> MHRFRVCALGAAFCVARRWRSGGGPGDRRVRTDWYRCYPSLMEEKDRDMYHCYYPYLFDHGDKMSLYPKIPDNPREWQVEQLQTTYDAIREDKYDAFVRLRAKFPELYQDTYAWDNPPPFGEFNMFYSVRFGMIGVKAFTCKDYDDLGNQFDCTAFWFPDNQIVKHSTRNGDVGTDKVYVGAMNVPVEFHKPHVAAFYKAAGVPVKHVSAGFPVTPDAYAPVGTKLDVRHFKPGQEVTITFQNTDYGYQGVMFRHGFDGGYVWLGDSKWQRRPGCMGAEGQKRIYPGHRMAGQTGASAETYDGVPVWRIDYKNSLIYLPTLIDADVGTYVKFRDTINTKGYTLWNEHRGTPPFPTFIPSEEEDLSKLATDEGQLTSPPLYMYFRDEFAAAQLVTQADVEDAKSAKPATAAPKKKVYDLKKYTEARKKYRKNLQKARKYKLMGVRTRAHEKQQEARRAKILKYKRVKT;> MLRLTQAVLRVQSHQKKRAQHPNAGTRFGRVYNRGFVRYGFGGFGMSVYSSKKDRTFKVMPVPPPPPATTAVEQRDDFADNRGLSATTRTLSPTFRMFALEDGGVLVSHPSHAQIMRWNQRVHTEEGKAANSTVMDEYVNSRIQAIIADNTIENTSLSQWRKAHMWNVIKSHGKLQRRWGTPDFVMGARSTLYNN;> MSRNGELCLQRIIVSYSPNKGNPAMRQFMATHLPEFHRQYPQVKIDIRPRQWPESSITGIYRDGSEKAYSIRFLSSMGINVRFHRLVNEGNDYNHSFSASHLHLQRRSVQGTWNPYLWNYEGTRARHKPPAQWSRKLTEKEWDYYVQQYGAQMKAEEDTIADRVRRYTDIPEASTEEVNQRWKEHVMPRLQTDLEYNLSHWKKQHRTGAGRPAPPTLNEYSLFSVPDHSSLGQDAIDMLRRREAQREEDWWRERKGQLKPPE;> MQPRRMAGHFNPTPQANSLAATHYAHTPELRHMADGAAMSLSGQRIPLLKPTLSKWSRQLRSDIYDELLKLPLRYALHDFRTLQAHIHAVPATATNASCTAAAGERLPPGVYHASSGLSSASPDAPAYYAVAGRDSAVGYAPPLGPADPVDVIPFFVHRSSNGHLPGKVYSMNAKTLMPAFYMRIQNIEGDMFRFEEELMKIFPTKKIFVRSHSVYVYNVNLDGRAVLHHWLLGLGF;> MTAPASHYTFANLKKLGLCAPQVALSRQPRLRPHVGHLNGLVYPLPYYAMWRGNHDKYTYNQATPARWGEGNTNTMYHQHYAHAKCPTDYGRGGREFQFLSVKRGKLKRKPLPTVQYVDPNSKPQWVFKSWHNPLSAPSMWEREVQYPEHTPAHTGAKRPLAVVAPKTSHKHLFLMHMEKVTVTVSPLLFGYGHTLQKAALDFYRRGLSARSPFPSDKMFLYYSIDHITPKIEVTWLDGSVYVPPLIEGVKAQDLIQMVMEQAWLAADRMSAEGRVLNPIAIDDYKWEQLIAFKQKRAKGAEAAKGGAKKK;> MLRRSPVPRRYRTAWRELLHPLPVWARRQQWLKRDTVEMNEAILREPYYRIKTFAQPAAFVSPRVSESAAHEPDTQQSSRYGVDRQLRGPRRAVSPERLQELREQLQFVGSIGPKVPPAAGAGTAYQDEYGTRLRPRYPQSWDTVPPHQPSRSEI;> MAFRGSSARLAATPGVGIAPETTPVKYVPEMLNIQNAKWWNGRGKPVYRSTYNEKSWLEKARWGAFTKGSRPVMRQRYSAAALKEALEMVPEGFETCDVPRPPQRIRAQSEGVVGRWYTNYWTLHSVRYQCQLAGVEWQFGERQRPRTNYDEPHMYTDFEETKAIRDYRSRWINVNRSLVGMSRRMKESEEEARYLHFKKVQDTFWSNRKVLVNRIKSMHNQGTLQSAKDLPIKTINIKAFLAE;> MHLHISSIPHRNSNNSKGGVLDATGPMLSAKRGALLLQAYHRPGEVISYKAGDYHLVPKKFTVGKRIAVRSYLDRNRTELSDRTFMPQKNWFRPYDLQDGCFDRDHERLSYRFYNLETKVIWKAFDTPELIGMLLHDETVKGNSGMYAPDMLDAALHYTREARYWRCIGITKPFYDRNTLRAHCWEDNGLQVGTLVMSQAMRHALMDLERAVRRKELGLEPNYLWDRWGPIGFIDGARADYLPRFEHNPYVDPDGVDVTEIDVLPFNTHEQIRERYRDFIEPDTAPFEEVFRSPSHGSLTTLADIPNASVVALYKDLKLKAGTPVAGDAVELAPADVRTLFYLSANPEWRAVADGKASWEEVVDAMQPVQAELDEKIDAARLLQNTRHNAERVRAFFEEKCGFHDFMYTPDKTITAAVLCYLTELRRICTETAWGAALAKCLTDMERVQGMGRDAFLVYRHIEDAILDKKRRLWAGRFAGESHEESTLDYLLENFGRRAERPRNVGTTGVEFDREQEPIGRQVQRRVLDSDKANKLAEIRRSRGKMWSKKRSVFDALHEKQLQNFNYGVH;> MCTRVFDVSQRFILLVSLPPLSLSLRPSCCSRKAATRRRRSTASVLLATDALSLFVRTHYPSPLLFLLLPNFPLPIHSPRKQMRAAVGAVLQPSSSVGALRCQARFITR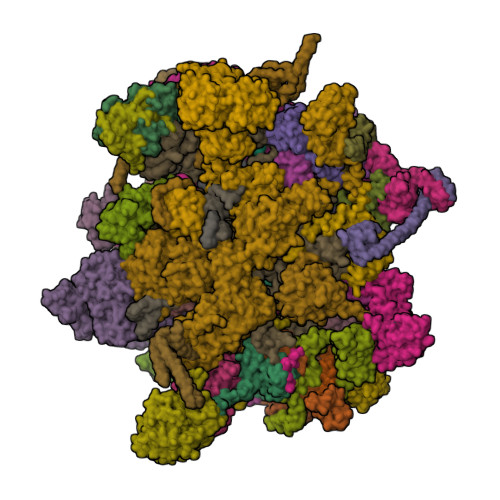LYTSYFKGELFPNQLARPLERLPRGVSLAAARKGQQAAAPSSSGSGNPATTASLDVVTWGDVDSTDLVHANEQSRAVAPQAGLAPRRPYVPLGEVAKLELQGDYLTEGGLHQEALEYYGVVAKAYELAYPKDHPQVAGIRLKLAGAFRRTGRLTSSKANCEAVLQMLDSAVQPPLELIVEALFELGLTSEAMSDAAAGTVFEEAVALVDMFHNSGQSHKMLRLLPRLGRRFNLNFEEKFVYFSPFDYDRVFALADQCLERAEVFYQARNDRAGVMRVLQQRKELIDKKFFNMRDFAGRIHTMRGHWKRRAQVLTNAPTPDELLRYSPTIHQVYRDFKYELNAPIGREKEVQPGVNRVVHDMGNPYRRSGVRSQRMFRDAEKNFEKYIRADAFEA;> MLSSAHRAAFARPTATLWASARSFGAGPTRLLLGLEQVQDVPTSTDRKPTGMHRGPGKRQTAPKEAAQYQFIKKWDLQMRETWDELEPFKGLPKPKVQFGNEAAEVIWPYALLLENVIKVHPYTKSIYVYYSQRQSTPLGELAARVAKRVSQAYLIPITFHNSHVYVEAEMLLEYSETPWVVVHCLDGTHKLIPVKPQAGQTVKEGAEEVLNGIVSACNEIGSAVKNPKEVMRLLSERPLQNQYVRVNYQWYGDTPEERMSHLVKWDYEPEEVVPQLRNRTQHVLDWMNYDGNLPTHNSVRVNIHREAARMRKPNVSAGPKTFFNSSGSRANARTARFDNSRSSQS;> MLRRTEIALKKGWTHNPGHTRRGGKNLAWRPKISDAKLSQFVPLALVHPRRHPNNWQERQFNALGYTKWPKDIGFYNAGDNFEVTPEAAWRLYVHARDEPYWGKLHCEKTIITLLPVVEKAPKENMERVLDVFRHYLKRYGADHYIYNAVMQAAAFAKNYEQAEQLFKEMETLGLEPNAQSYVNMMLAAKLCGLPPEKSEAYFKRAVKDGAMQSVMRMDTEFRMWMDQLDRLGSFTASSGYLSVNEEGAKPMPRDMWAIWGWHRSESKFISRRDLIMQQVRARVHSGKELVGTVYTKTRRQPWAKFNGMLRHDYNGPSYRAPTIFPDAPEYTNEAGHKAF;> MLQCTALVLKSQHKNVLRKGRPHMQKYKELNRWQREAQGITKWEQGHSHRPQPYVERFNPEGAGLTRGTSAYAWKWWHTQYPWLPNVAPADYVPPSPRGIRPAAWDDEFADVVLSMSDEEIQSYLLDKLTEVIFAETQRDGYELRRLDFEGKPLTELPERRIIENFVFEEETLRERVLDRVVEGVFRLVPTSTDRLELKSVANIIDFVLTHVTVARKPLQHEIPEAARTVMRSHPLQPQLGFVHALPTDNRDAVVQEWERMHHLDWQFGKAVYEPRSAENERGNLTWLREVRHHEAREAFQADVDSGEARRRHMAKIKAAAQVPHTGTTSQ;> MQRCLARLFQAGVHTPHGSRYNAARMKNWPVQEVPQNFNFTNEQRFKAKAVPRDTGKIPRDFLLSVLYRNQPCEVASLWEHCLHDPQIVLDSKRHLREVLQQARAEGFVSFEKDAVTDRWVCHLTRERFEEVRALVGARAEAQDLYSGLRGASATETSAYSESFREMNEDTKREHFRLLSEQVADTTTHLRKFQRMEMDYLPYTDLNGKVNFMWWYEMSDTRDATALPEAAAEGSPKLSE;> MLRWSRLLREMAPELQLEYIPIIFTRTILGPQGGFAGEERLIKREVAQKYMSEGNAVTPSAEFHQGVWCYNPDSEQYDRFVERNAEFLDFAARKRQWLDVYWRVNTGYLLFGRQSWGQGWLLNCPLRKKDIAQKLWEQYKVRVDPRLIEFREKDRRTGIQDLGHNWCWLYLPGAEELAIDREVYDNKRVKVRMHIRKMSSYGALY;> MRRLPLFCRRPSRCCGATASGSGSSSAAVLAASAAPSVLVLAARGIATSGRVTNEDRRWWLVHLECAPDVTPGTFVSWLDCCGTHTTKKLIERNIWTIEQVAELDSDRVDELKYKEGCLKMDVVWEHARTIITPLKQREVSGGVESQLQSRILELRKKRELERQRELLARERATVSDKREETLRRLRESVAAKKAALRKKLDEQHGEATPAASESASTEAHRGTAEAAVEDEAVGNIVDRMSGGNPPRA;> MRPSALCLGGFTMKYKRGTGLWDEDHVNDFDANKYLSARSTMRWYYGMERLQTRNNMNARRATQSYNNNMGLHHSGRGAFERELERRGIQVDKYPLTTTTGAARVAEMVLLRRQELEAHAKKAMESQRQARRRDAPSEWYDETEGPLNPRFLASMQSNYTQVITELPSSPVTGRRELPGASFA;> MMLQHTSLLCRKALQSYPVPPRARNYERRWSSSRTNPYNRMFWRTVLNEDFARPSFWVSDFRHKYLAKHGMDYQGRVPASPAPGMYQGFSDVHKILANHPKPQRESRHLPVMPMTPRVVFEHAQEKRIDYAKKMHRDRRLVEQLRTHEFWGWYMKLQRVRGRWCKEHGVSSRGVYGPAVDAAELWG;> MFQRTCTPRLLACTSALLKRSGKPSDLPDYKQVYLPYDTAPTKTELDRERRKFMHAYSGRMEHRKMVEVKDVPQNMYTYGKEGMSIPISIFKDQADPVIGPEWTYPGIFENKIVAQHWYMEELFDREKSNTFESPWQRQVLDNQVKRRLGKVAWRMSMLNIKTIDIFHKERGASKRPGAGDTKAPATPAGKK;> MSSGAVGRGSFHSVVAGANPRRIPTYYNSAYELIQLHRAHREVTRNFLVRDKVFDNKFPGCSLANGLFKMVPNKRGNFHTRELTESIRHRTIWGQRIQQQRTINAAILEDATKVLSPAQMEDRFSYRTPDAAAYFSPQEYTAANNWPNYWQHPTEKHVVPKPRWRREPELGGITRVRDAVATPIADY;> MYFYRRIPSLASKMNHMRQFSLPRSSAAIIMAASTAALAVPCRAMHGKPASGHKVRTQHSRRWWMQSKAHHLTAVPHEEARSRPHFPAYTEDVDQPMVVPDGVCCFNCDKPIDGDDINSYVWVPSGNARVPTTQGYFFHVKCFKCWNCKYRIIHNQFYSKDSRAWCLSCALGRDIRVPTRRWHTSYVNTHRTGSRLTGQFFPRHRHQMEFLFSPKE;> MLRFTQVIRKNPVVFKQGQGMFSHQLKRILNKKSLHKYNWDPLHMYDPRKLVHANRYVDHDTYEEKYDPHWEHNAHLVPDQQFYNIPVPKEYKDAYWWRDLQARRVQCPTEWVHFRMHTKDKLKYDFQDLAFRKKFEYSYEDVVANAKDMCS;> MYDSRSSGVHDVAPRDGVDFMYEGPQQVLPGAHPLPLFHPDNSVTRPPVSPYLPSPQRPHPYFTTELPELPHFQTTRPIVYTVGTMKQRIVAPVFDLANNVTHTRELDPFIFGFYPETEEMAKNLSYWLVRCQNFSSKWDYENREIWRKAKKNWPNTGMGMARVGDRKNHAHPWGAHSKPVKPWNLLMPTMDVKTWSKSNRMLVTLKMLQGKLQIVERLTLPEPTQEAYLQLCRTMGWDVRHKGGGALFMDGGSRLTPSSEYDRAFFFGSFFNGRNKLVRPTLLCDEPYDYNRTSSKARTKGPKGQKNPIPINRFNAYDALTHDTLIITEGALLQLEDEMYTHKLAMLPPHIRAQLPERGFLDSEVLGDVPPALQTVQMEAAARTEEAEQAMYAPYYDNPYHPWQDEGEASYAVDAVEGTVQRYIKSRKTSWAMLS;> MAQWIPKTAWKVSNLNKRYGAPYVAKGYASLDPRCSLDAYSSFQQTVTSADMKKALLSIDSTSSGALVIDVRSEPERRLRPLLSPAIVALHPHDILSGAACPILPSNKERAEMFVVASEAQRAVNACTALRRWGFSRVTAVSVDAVSEAIAAVQKPADAATSSSTKS;> MLHRSCVLVDSFKEHYHRVHLPRRLALQRYIKREEARLSRHKGKAVAAAAAAGVQPGEVAYKYNRWWVSNDHEFVHQFAFVEDPDVTREKRNTLPLVTKENIWKEPQQTFFLPFAPFVRVVDYAKDPDTKFLKPVNIPRWKDYMQRTKPIVPRTWY;> MLGGLRPLAAATRRTVGGALVSPALITPSRALSVRTEDFFSKEAVSHARRVSWAPHTTEKKVGAFAKLSRSNFNDPLPVSFQSEPYFEEEIEAYRAHHRPDVYVYKYNVSPTHLSLRE;> MRRTVRALYNSFERGWKDKTVHPLDRRGRFNLDEAAAELQLDEAYVASLYKPLHYTYSMKGQRYPAEQGRTSRPGSLAASRDRMFPLYRRNYKLNRELRVLDHRRISTD;> MLARYLDPSVHPLRVGQVVAYDYLHAAKTWQWTLGTVREIKDYTAVVQQWGLHTGDIDTLRSILLKEVDTENGRMKNYHDMLAIAREKLASIRRSNEDRVSHVRGHFDKAREKVELIDEVDLRKVTAQAAPSPVAVAVLKAVWAVAKCDPTAVEFYEWADVQLEYRKPAALDEIAKTDVLAKLYPSAESLQQSLEQDPKLNYKAAARDSPVVASLHAWVITALAYQQAYNLLAHDKRIQEQNDAIAAAIAGMKACRAKIAKLKDELSSKDTAALPGQVTSFTRTSVLVTIPLSAVISPVNVDTDVKRCVLTKDEVEQIPIDAKITRYAQKQKLAITGSHLLDQYAAATTTHIYVTELEDRLFFFQHYMASALRDAQTAAVDAHQRLAVSLHELEAFRQKRHDAKKARAAEPELADADGVEPSSGPTSSRSPTGRAAPRGQSAAPRGTASQQHKLLGPAYQSIDPATIANEPLYAVTIEEYKAKDAAGERAMDEAERMADEVQRLAVELEDAKAAADKLAEELAAKDEELAAHRQKRHDAQQARASDPALAAADAVAPRSGKGAASPHVGAVQRQAVDPATVPVAPAVIAEEPLYVATAEELQHVRDFADQLAEELEAFRQKRHDAKKARAAEPELADADGVEPSSGPTSSRSPTGRAAPRGQSAAPRGTASQQHKLLGPAYQSIDPATIANEPLYAVTIEEYKAKDAAGERAMDEAERMADEVQRLAVELEDAKAAADKLAEELAAKDEELAAHRQKRHDAQQARASDPALAAADAVAPRSGKGAASPHVGAVQRQAVDPATVPVAPAVIAEEPLYVATAEELQHVRDFADQLAEELEAFRQKRHDAKKARAAEPELADADGVEPSSGPTSSRSPTGRAAPRGQSAAPRGTASQQHKLLGPAYQSIDPATIANEPLYAVTIEEYKAKDAAGERAMDEAERMADEVQRLAVELEDAKAAADKLAEELAAKDEELAAHRQKRHDAQQARASDPALAAADAVAPRSGKGAASPHVGAVQRQAVDPATVPVAPAVIAEEPLYVATAEELQHVRDFADQAAHDAATREAEVAGTVENLRNELDDVREMNAKLEDEVFALKEQLSDAEDAYKKLAGALVVAEDERQELCDDLEAALDELEQKKDEYDELLGNLEEVQGLLEAADVAGRTAVEALEQRNRDMADLQGELANALDASKENENLRALLDAKEREIDRLKEYNSFWTDTVGTGKQKVTHRLTKIFDGDWTRLMRHRPEALKAAFVIDSSNACHVPGDQIFLVSNSFTRRLLTRTDHCPKCDRLSTFRFMSVSGMVGRMPYKPVDTPGPSYATLYWRKQRSGKIASQPLNEVCNKNEF;> MWRLSRVALQSNRAALYMPYTPVATNPVVYFDITAEGDALGRVSVELFRDVVPRTSENFRSLCTGERGYGQCLLYYKGTPFHRIIPGFVMQGGDILTKDGRSNVSVFGYPFPDESFEGKAGKHLPGTVGMAHSGPNQNGSQFFFNLGRNEQLDRKFVVVGQVLGGWEIVNQVVKLCGSRCGTPVSRAWISDCGQSGGYMAEETQEALQGERAQHVIPGKEVLDLIQPRY;> MRFDNAAPPPPPPPEAAGSTTTSSSTAASALPRVSYRTLPSSMYPKEVSSDFIPFPLPKHDASMGFGPVRLRNVPDIEEARARMAKAAQGPPRGSASTQLQDADGDNAEAASALWAELSGETTATSVGLSTTSVTGASPEDPEALSRPPDAQDEDLVGYHVHRHFPLLDVLGCDRSVNDLLAQFWNRPQREARTATVLDFAATLQRHSNEELTRVLYELSSLFEWDGNGLQFIAAKVLKYGRSYTVSSELTKAFVQLVDAMTVAFVEEQPHRLAESPALLAQVLHFLALVKIMEPNKWYTLNPNAPQNRADYTHPRGVNRTCGHVTTGRALLDFLEDMVTSGHNWTGEAAVDDQQGSLARSPVPQHATNRFTEGWSEDDILDVMAGFSGVMPDGKASSPVLYALLDELWMRWSKVGFVLSGSEQAVRLERLYMLLQVMDMQRDAVLDALLGGQLRAHSTAPSTSTLPTLFCERDDTPPLTLAQSLTQTRGPDFFSAVSRDKRAMVKAAALRLLTASLAKARDDSDAVLHQALVESGTELLQSLTSKSAALSFAQREQFDVITLRAVPHMADVAERLAEQRAEAPFFPLTASAGGLPDTAAVLAHLSSHPAPYIVLCKGRRVHPVRTLVSNLDHVAAVENVFLLHSSGVSKCVDALVAVARRLRSGKDALIVTASCLRALQAAAQYGATEKRRATADRALDIVSYELEAGRAILMPVTDELYLHDAGTYCDEDLMLWTLAAYLARDVPLVKVHTIMSSRSRARNPQHALRGEHSPLTSTDDLYNKSTPLLQALRSKELRAVTHHPVVQRPVRDPPQTLYNVNPIRARFVYRRDKALFDKYHVTARNLAPGFSQGALNSDLRALGFYTPDHPQVPYTPLSELKCHPVPANPPASQ;> MSVFPGLCGDVATTNYRVFLGTLPNLAVEERFLRQVQPVFPWYASRKHVKEQASEFLEIDLASCDPELLLRYTHVYYVRRQLYDELVDRQLTLMETGKAAKVADSALLTCLAQVNAAITPRLQYELHLLQQAKKACRVPRRRELNPDAALEAHDYLCMMRVVEEDVGGIPDAEMQARAYLPREVLEAKVKELAAMIFGDGGSATKGTGAALERKEQKLLQRMIPADYNKVGAVEKLRPVDVTALYRFTGERVCGRPADKPFARALWGHVFRKVGSHPLYLQRASLYWARHSGLDPQSATSAMPADLATAVCVQQALFPALKYRCQYLYTSPDIARQQWRTGHVVPLLRLFPLLGAPAAEDLAAQLVVEGEWAKLGIEADTNLLHDTVLRQLKDMVEQVSALYESDAGAVLKRVEDGAKVLCPSLSERESLTMRGAPEDTSREVSAAAAARVANAAPA;> MRAAPTRLAPSTVASLGRSHCGSQAYHLDAAGAAGWRRRRRLTGVSMTTTHTVAPAVSALPFSLSTARRTYYWPYPENLVPEGATTSPFQSSPVPSVRERIIREYALGPLFGSRTPCCVLGFAGTARDVAACKRDVRRWVARALGKSEADVELGALVQAKEMLLHRSGTDESPRLGDGPGSRPDAEQRRVTRYARLPVQARTLLEVYLPGEEHGEVDAAADADATILAHGYFLQEQLHRHMTTTASSGSDPTGRRDSEDCQPEEPARKMQSHCQGCSEPNDEADVKSSVAALHDVCGVIYCEVPVLDESDFAFDQLCGKEVDDETTERVTDRWTRRAMQQQPQL;> MLRFFRARLAPTTTDAAAKLPAGNPVNKTWFRHNLIIRRKGSYRSRWGNGTEGYGAGVPLSDQVKLHCVDNTNCKHVRLIAKATAERFAHCRVFPAVAHRVSVQRFKGRGGGGEVSRHRVKPGNIYWVCLFTRRQTNTRMSGLQTNFDRNTCIIMNDQRVPLGTRVMYCAGRHVNHKYHLKAVVLANFFV;> MRRRDWCGVCLPAATLHALARRYSEYRSSYTGARSAPWAAPEAAPAYPSARSPFPLERPRFRKTHIEWMLHHGHGDRYGKYGPSREIADFEYADGTPSSISGKRFALKHHQDHLLVQLIRSAAIVERFEEEELLPRIPGTPEQRSWDPEIPLFLEDVDEFGRPPRPVAGNMVARVIEERFAQESGRTPVNLANKHAGEVLEPNTMFATYDPAAFVSDDIKKDVRRPFWSRRRWALSDNFMVPMSPKPKNTIKDE;> MLRRQCVVLSYQRGSWAPGSKHQKHMSLNPTMYLYRFAGPHGPGPYVMKYWWTLGCFPTGIERPFRLPEFLASYQQQHVPIEVEEWLQCFVKNPYEELKDATSSLLKCLEEVPIRENTRGYRSIESGVSSFAAPLAQFERQLNVRVPSLAVRAALGSPALRERLKDDLFEYNESLSACGSTPHRRLARLAFDEPLTLPGGINNSDDSENLRGQISVPMSEAIGSYASPNPSTSDDEKKLIRLLTTFSEGCTLKEDYESAFSLLSSSLGFSHDDNTDGVVHSNASAAAILGGLYKEAEFHGRQAALLEPQAMSSRKSGGRGYVLWATATAYQEDFDRASRIVEKGLEVFPDNADLKSIQEKLAGAVPAASSASPLCTRMVRSKGQQARALLHGSGRSFDNEFDWVVFKNKLYPSKMNPSSNEMGSVFRRVGDFGGHISTSRSLEPL;> MILITSNCARVAAFARKAACRGALCDRHRCISGGGRGDLFTRHASAFKPPAFGVLRGLTHSSQTTHPQTGQLRARKLIQHAMHDRTLSGSGHHRTAVATWSYLLPSLRQNVEQAVPDTLYEKLLTDEVPLTPAESRQLADAHRLLRFELQKRIGLLEDSLADAALPYLLQWPALFQRAWLRLPMDQGSASVTDAKRDAVVPAPPSFVHAPAALPITEWAPTLSPASPSACSNGLIGRGALVPRLAQLTRHVIRCVEEDLGRLEHGSEPREDGAPRSRRQVTLEAAWRAQWASLLSWHAGTS;> MRGAPTYATALGSACLPFALDCDAILQASRRYSSTSAHGARSSAAASTSKLNYYRNLGVDTDATPQEVKTAYRQLALKYHPDVVEETHRAHAEMLFRRVSEAYEVLSDPVRRRAHDAELGIQTRRKQQPSATAPAGAPSAANAKAGTRAGSPAGGARPSSAFAERRKHTSSTASSTSSTTFQQQQQQQRRRYRKPFVRGDANRVFSDAFDGKTLDEILFDVQRRRRQEKAGRVAAERRHEKGGGAGHAASNGTTKSSSSPQPLMGESGPLDHDARLRHVMETAAELFAQRAQRQYGHGVLRHIRGVAGPLPDGPAPPPEVYMPFRPFVGMPVPPGVRTPPEPTLGKVLDSQEATVDSSSTPASRDAAWYEIPTQFHTHTYADGTPQSRSASLAKATKYIHGMPHNMGQLYSYHRPY;> MRATLRQCNVFDPAFMRKVKRTLSAYKGSMETSAKKSMSREAFVDIDEKGAAWYLGHMQSAANMLADKVKDADFILEIRDARLPFTTENPNIRKLTAGKPRLIIFNKAELSNEDSNRAIQEYYERNGAFALFTSARRCWRDVVEAVQRFTTHILPPLPYKTVAHVGLVVGMPNVGKSTLINSLRLAHEYQFHREDFRRSRSPETVSITPGTTRGMKLVPLSKDPPVVLYDTPGLTLPGCFTKESGLKLAACGIIPTNDVSLPQGMVARYIYDILVASGSSEHMAECLHLPRVPISFDDCVAMICERSGTSGQTEMGNLDPVRAHRFFVHDFIMGNLGKITLDVLPRRLLRSSQSSIPLLESGSSTAATDGAQAAAGDDDGYAWTHHVETSDVVERYPDHMRDVLQSLKGPLHHDGVPRRHQAPSVKNLDSPSDCTVISRKKGPISRVTAFDEQLKRHTRLTPGR;> MEDTARTDEQRRRVAGWTPVVKTLGDHRLRVAIVGRMNSGKSSLFNLLCEDPTMPAKKNIVKDFNGITRDCVEAHAALDDLHFTVIDTPGLLGGKLVEEAFRTVETADAAIFVTAVDEDVSAEEHDLIQYLAAKKMPTCLLVNKMDLVPEEEEALVLDVYNRLGLGKAVPFSARKREGLDMLSALLEPLYHIHAMRKVENDWDIEDLAMAGDEAAMEEIRDRNCTDRYIRVAIVGRTNSGKTSLVNRLVGYERNRAADESNTTRDPIEIACMYKGRKLKLIDTAGLARQRYRTDREFLSRIHSLSLNEIRYAHVVIVVFDATEGHPNKYDMSILHKVAQEGRPFVLCANKWDAVLDQSATAEAIDFKIKRQVQEVKYSNAVVVSAHTGMNLTLLMDQVLELYDTWNKRVRRSELTKFWRKLEKSVIIPYHVARVGRITQISTRPPTFLLQLQTKKEESQLPKALQEMMKNAITEEFGFRGVPLRLVQEVKDSNPDYI;> MSFATSITCVLFYMLQLSLLLRGALCISYRALKSAAAAPVAAAGVSAASSRLGGAWEGSIERAEALENLSNEVFGRGNRHLKNVETLTALPEGLHSFPEVCFIGKPGCGKSSLISCLLHNHRLGKAGATAGTTRLLQFFNVGDALLLVDTPGYGGWRGREVGQRLAEQANAFSILFRYLALRNGSNLKRVYWLMESSAPTPVSFQPRDEELLTFLSRERIPFSVVLTKIDRHWRHYAEQQRTADRVGNDGFVHPRHRRPETHDQGFFTRTSLPQDGVARNMQEVYEFLGTDQVPILGVSANRLQPNRSRNLELLQHDIVHYCTQDLLHSEELSFRNMHKLSYAPPTADRIHEIQLRYPVESFVVPENNNMSLARMVEHHEEMKARFCENNVCARRLSAKDVAACHLESVAKLKAACKHDTAERERAEKVRPTATYLFESTLAAAVTSLPLPGDVAGLLRASEAQGTATASVSRVGGLPERWKECDDHNAEACAADVCASRRFRVRPLLVGERQTSRDSLGDILERALDEEEPRQDFAGSIVDKGEKTANAASPPHCAHAETTSSSHTLNPVPDEAPVPQPYRVDAVLLQEQPLEALPLPAMLDPDAHYVTAIDGTPIPRSMISVSVEQLAVSKDDELAHFATKSGAGAYEELIVADQEKSNAGADLFMETSDVAHLPEEVQTQLEEACARLTRSAARKQKERFLTKYVERKRKERSIYMQAEGYMCPWLGRSEGRSVVQGFAGSCGTGKGGAVMRDLKQKGFGGKSYSARTMKNRGRATKKTGFWAA;> MAVASTRLPTVGCSCSVATLAYSRTYVRSSNTRSTGSSSGSIISSSLPWSQHRCQVRTLIVPRQLKAYGGTFSQSIGERVDHAASHQVLQSLSPARTAQSPLLAKPVKTKVVDNFADMLVTPALQEALADMGVSTPSPIQQTAIEAVLQRKNTVIAAPHGEGKTLAYLLPLYQNMEKDRDVYKIPLRERRPRMILLAPTKELVEQLQTVCARLDAATGLTSVCFTSRKRSKYHLSRMLKNTMADVLVMDPKLILRLLRTRRLFIEDLRYFAVDEADAMMSSLHDHDAVQLLMKVQKRNQFKYLWPVQTQYVFVTAYMTRKLEYIVGRKISDPVTCMFRQLMHRPQARLRHRFYAIRREPEKFTVLMHLLRKNGHVPLPIDTDVAEVDVHTNPRKLSGSLAEWHEAVQRCAWKEQHEQEKSSGSGEAVTDDVVDVDEVAVRAPEEASAAVPSVGLSATENAAADDDYDHDSYARYTLERVRPLHWEHLTTVAAPFTCPIRRTVFAEGRRTIIFFRNIDATTAVFHQLRSAGFAVSLLHASLPYKVRKEMYADFASGRTNILCATDVAARGLDLHVDMVINFDVPTNALAYLSRSGRTARMGREGQVLNLYNKHQGVIVSAIKAFLKDNLPMEGLTNRKADMMQPRYAEWRTHKINALARSYVSLITRKTIPAHLERTYVHHNATWRPVFHPQKTGIHGGVAPRQQQKLMDRVREQAVWFRRGQLARRKGGRAKFGSRTMKHGVWNDIGGVASREVVNEAQNPSPAGPNFGPPSGPPQ;>MGEQRSVARMSKSAYRHPLAPKDPSQRNVTIPIRASRAAASASSSSASAALSAEDLKKQAQKVLLLQMQQKVLWEGTVIDDVNHALVQHFLKLSTNDKYRQARQMLVIGGRAMIEELCRAGHRPRHLMVECGKPIPEFLHDRRKTDVVLVDRSVSVAVTPGSDGYVGDFAIPTPPMKEKLIANHQRLNRVLVLDNIEDPGVLGTLLRTASGYQYDAIIATNHCADLYDHRVVRAARGAHFQTSVPIYTLKDEDGDDVYGLLNHIVERNNLLPLCYIAQADAAGVDGETAGTQTGFVSSPEAPVGRVFRSSVVGAAPVPLPAPRQSDSSYAASLSRELASVSQAREELLSDFCLDRFTGASSAEDDARSGYILFAGPNHKRNMLRRLERSLSRRSTRLLLDSLPSPSEAPSDLLIAMSVVLYTLRPRGNWDYLPVDTKHEHSTLDLQAKHASVDIGVNRLRVSVDDINLDEAEQQDRAHEANEFMRWRRLARRRGSDYDHWMAAEQRRVQAMVRRERQRRVAPWMPLRDAKTKPMPDWVPNIIDEYRQSLDRDALARERDISTSYQRPPR[2x];> MRRLFLLLAWQPSFAKHLSELEPVPQRAPVEKRRRQHIPLSLQAREELSRKSNELQYHVVTQDWFGQRVDDFVTQHHPEWDYETVKRLVQQGHIYRYRKNGKKRYTRLTDRLEFDELVVVPTASFWERQLAPPSGVELQSSSTSQQQERRQKFHLSAKTREMAQEMVLFKNEHVIVINKPSGVPIMPTHDPLAMNITDLLPAWRYTNTQTPVICHNLDTETSGCVVLARSANTHRMLGRMFVKRVVPNSVYWGFAVGKPPVNFGRIRMHFEVQKGQGGDVIVARPTPTADSKVGIAEFVVNASALEFGSFISFYPLTTRRHQERIMAAHALRAPLLGDAKYGGESAFPHSLSLFWDPARKDVPLHLHHRKIQLPYKNGAGEFVCVTAPLPPHMEKTFKRLGWPVDADDPLIPG;> MRVWVLAPHSLPPASFRPIFEARPPSSPTHSFHLLPTPIYLYITCTDAVDLYVCAVTSLLAEWTTTMFARSTIRWAAGAGHAFMDIAIGSQPPHRVTFELFTKRCPIASENFLKLCTGENVLPQVSSIDGIGEPSFRDQFLPQLTYRNTTVHRVCKGYLVQGGDIVSGQGTGQLSIYGESFDAPEEVKASKFDRMGLLGTAVSAPHLNGSQFFILTADKAPHLNGTCICFGRVVDGWTVVKAIEAIPLTAAGEPAERVVVVECGKL;> MRRSAWVFVAPWVPPPRHDVKVTMPPPPGGEVGGSYGVSTGYSDRLARTPYWKRMALSTYALRMKENETRYPMSPHREGEYDLRYTVTAYPDHIKHRPLLEIGEAHQIPTIEIPVIFLVNLWDEERLTWFGRQYETVYVNRNVAREELLPQRYAIYATEEAYKLLGLPVVNHSIHEEIPKTPHAYKKLLEKQSYTEERWKYTIEYLFRKYEADPPELQDKSEDGWDGVEELATSATAGGAGDSLAKRKGPVKQRKARKIKLF;> MKALGRGPITRLANTAAPGGFAAPGAVYNRDDWNAGRDVSAEERQCGILTRLCTLAATAPREAASPACGLAPLEAVIRVQSTDAHVTEVDANGGGAFLEKAPKGRWRKISRSKTLLVEDTATPFSNSDKSFSPRVQSYGEYVRRIGKLPEGRPLLRFAMFRDGYSLDSVCHRLRYEIGVPHDGVYLHEPPGGSFAAVTQFGVAVGVTREQLPHASRHYNVHALIFDDRGYHALDELPRLSVAPQAYLHRILLRCVSGDEAAVAQRLRHLSSNGFINYFGLESFGIGSNTLFDMAAFAFRREPHRSVGAYLQTLAECSPLHHQPYLSYANAEESTVAGAVAEWLRVCERAKLPRETRELLRKLHCYHLSQCHPSDATTISMEDVWKACPIMHRAEQSAAAFVWNAMASQRLLSFGSRPVKGDLVCRIGNRGAIEIAEVASDTDASHYTIDDVVLPIPCGGTPAAELRYPTHSVNEAFFTQFAKKHSLSFLFNSGVDPTPRAAATLGPYRRLVSRPRNLQAAVLQDPSSCAALKSDLFLLQEHQPTEGWSLDYRQRVREPSNFNVSERFRERMSCIRKRRAGEHSVALAFVLPAGSSPWVALREAFHMHYGTFHDFYGVS;> MIARDPPQEGRLPDPSRLPYDDERFAEMLLEMEVNGVIDETWQDAKKARMEDVKEIANILSSLKVRDLCCVDVSEKTSNFDYMMFGTCEGARHIHLAAWAVQDADKVHRISKIKRQQTDELWEVVPVGRIVVNLMVESFREEMTLERKWAVTRSMDPLAAANAPISEGRQVKAHGLWTLTLNLQDLEDFEVDYCKDILMRQM;> MQRQVIRRLGNRSAFPLVAAVARSSQIRGAVRGDSGSRARVIPSFMCSLRAYSGGHHEEPSSRSGQYLLDKSDVLTRVLEVVKNFEKVDASKVTPESHFVKDLGLNSLDVVEVVFAIEQEFILDIPDHDAEKIQSIPDAVEYIAQNPMAK;> MPLCASPVRLQLCRTPSVLGAGGKWWKEGPPDYTRANRRRMELEQQRIESSQHLPPIEPTAEQACHLYRRLLKEGYKTLVVTDKDFYRRKVRYELEVTSRQTSSRVRGIMFEKGHWMLENKLGGII;> MLRRSAVRYLKARPKTVNIEPGSNRFLDPNVEAKAKDIFAVPEFPNKAVLHNWRFFIKAGKAATGPPVGQEFSKLGLKAMDFAKAFNDRTKPHFKDDIELIVRIQVYFDKSYIFRIEPPPTAWFLLRAIRKKRGETGPVVLRGNYCAYLTLEMCYEIAKMKQMSWGKVEYPPIEVRVRRVVGQARRMGIAIIGIDTVHSSPVKGMTEKQYLEESEKHRKVHMIQYEALKAKELESAPLIERLHRPNMAPLTNTQLEEGLKDANLLNALWKSSHPKSLFTQDTRDREMARRYLNTRGWFKEMTPEEMRVVFLNYRLPKQEDHQRQLNMTNGQAQSQAYWSRDAASPQ;> MSKQWLCREGERWWLLDARGQQLPHVAKIAAQYMTGQHRPDFTPGMMTGDHVVITNIKDAVMTGDNWIRVPITWQTAYPGGKYRVRLSEMYERDPCMVMWWYLKDEVNRHFVRKLKTRTAPLEKAWLYEDSVHPHAEKNPRPLVWTDTATMGWRYKDPTFQRRWSPNQFMS;> MLSISAVQRRYRLFHPVHQTVPFHFNPVQSIFPLIYENNLLAKPRLSWKDYEGRKEFDADHPLPVVGTRLNERTTTHKWSHWDQYINPQITQSWMYLTQTPEYVGPRSGHNVIKMGWMKIGGSWKYSRSYNDARRGFAKGQWQERKMTPRFMLAPRVSAGGPRNRYEGKASFSRLSLSKLLWAVDTGRLNPNETITLYHLRNAKVIADREVVWPGMVLLAGNVERVPYPLHIELQNASAKAIQLLEEAGGSFTNVYMSHEGLYQELHPEEFPTFMEQELPERKGLENFATNSRKRGWLAQWYEDESRYAHPGAGRRTAHYIRPPTDRDFPATIEEYELAKHHQKWHLNQPGSATVLPWHSLNTADMARRSAGRL;> MLRWSRLLRGRPPPVMGHAKRMRFAGVDDNPSVTHKPWDTSEPLMADYGWERGKLPKFRARSPFHRQQIARRMVTELIRKDYVIVGGARAPALRILADHVVELAKAGDTDSRQQLAYFLHDPLMVDKAFDEYPRRFRDMNAKYAMMTRLKGRRRSDNVAMYFVEYKNRDMSDNHKGEDYTAGPERFFLPPRIIETEKGIQRPPHMQMAFDRWASKFKTEEFHHWWRLRHAKLRYWGVRNVPHPSDVDPLWTEKEEEEWHNEMLANTSDFEDFDLDDDSYEAAGEGGSQGGSSSLSGIGPEPQKKY;> MGYTRERTNRHFFVSRANAFFSRLPISRIQRALAMEAIKKGSMKPWKHTKEQIIGSPITCNFEYNPRPVRLIGTVMDAHTEETSIKGGLKVYARSEEANMMLWIPAGNPKLKYEVTAAKGSFEHYLDERSKWDEAWLTGRARMK;> MLRSTGVSLYYRATAELDRLRGMLRGRARLERKVGLKRITFLMRTQTRYRVEQKAHWERAIVRKNVDSAAHEHGSGWQHLRNDLARQNLMLLPRTQQQLAQYEPLAFRAVMELCASRVAPPPPPMTAQVPEEAYATRPEDPKVAHPAARRQLEECVERMLCTGRSDVLQREGPRTTQAWMDAWKEYDLGSAAQK;> MLRSANPTIAKALQPLIEGPKFAVVYCGNHQYKVSPGDVIAVQRLRAPIGSQIALKKVLMVGGPRFTAIGRPLLEHVRVTADVEEQKRMRNVVSLFSTPGRRRLRWLDAQHAATILRIREVVYEPTVVGELDKYDGVLLKDFHADRHPNPVFTANDGYDLYYPKDWNKVEEASAFLEMMEAPPTEK;> MPKPAPRYNIGLRPAPKRQNVGGQFLATQKHYARELWYKRQYYSTRPFAIQKHMGSTPRILLDRTLWRSCWLTKSNLPDVNRWEKVVNSQRVTEDRWALVEEDGVMYQVNWKMYCERLETELQKAQDQLPQYSFMMKAVPSAWKKLDIELSVLRGLSVREAMAQCKLSPRKGHMAVFRALEVAQQGAEGKGLDKEHLRIAYITCMPGPTDKQVDIRSRGYYAWKTKKSSHLLLTLAEDPEMVLPDRTAIPYASLMTMKRAGLRTEPTMLDVPAITAEGI;> MKRLSSHHAIVCGAASATAASTRFGDVVGGGSSCTATSPLFAAQRGRFYRPLVNQGINLWRSRMGRLHKGWTTWEYNRDVIPDPRPFPEPAVNNYFGRSRIWNPIAGKIGLVNRKAEEWGWPHQRPPPTGLRRSPEYFPFFFSRYFPDVEVRLVLDSVLNNETTRPIFHIPQDMSKQELVNYLKNIYNIDNVVRIRVRNMRGRRFKNEVGEIKSLPDYKVAVVELDSPVSIVFKQIKGTEDTPDNKPAAQIT;> MGCVRVRTGCRIRCVRASFTYTQAQMYARYRTRSRFYKRPEKMLKAYNVSPNLLRLPKVKPGLLKGIYTDEKIDLRDRERLELVESIRHPKERDFYQDHTYHNQWIARDLESHQKIQIAGRYPYFSPDYEIKPWIWYPGDTVEVVSGEGAGQRGAIIAVVKYKNEILVQNVNVQDVVIPASETRPEQVVQREHPISVLRVRHVDPSTNQLCHLEIVKVRNKETGELEERRISLESGALLPIPAPEETVEAGDPLKDTAIQDADEETYDREKEMPLLVVRRLQAMENYFVDSLQKSHEYHKALQMRNAQDMQTFQKDVLVRATEKLAAAAAVAGHGAMAEAGSQAASVATESSQAGDAEEDAVKGTITVETVVAEVLKSEQRFRSDAAAPGVPGWWQNMIDAYVSVLEEEEATIEAEAAAQAQAAEADRRAEQLMADATAEAGQSMEEDGTMEGGDEDLDEQDGDLDEDASRSDRSK;> MLRQSSLLCFSTFALNPETSRAPHGPPRGLINRYISMGLPPWAAWCNRVNRHALYRMSDVSPRSFLPKAPHEMDVIWMNERVRERVRTSRQVQHVYRQLKYPFVKTGIHYSDTLDHWVQVPMVEAAMFEIEKDGGFDNFILKRSGPELRSTYGERIRRHLLVRQKETQKNFVLDQQAKALAEVTQAELMKATSEEELDAVLAKYGMDAEEFKRLMAKRVMEQRKSVAAAGLRSK;> MRCSARRANVAALYEFVDGNFLNNKRPAIPGGAWPLESLRRKSLADLQQIWLSLLKERNMLSTIKEHYLRHQEELGAMPAPSRLKMVEESMENVKRVVKERDAEATAEAVRIFKERLAKGIYRYPPGPPPPPGAHDPTSTVKLVLSRRVDEERLRELLGRFNVFEAHKGIVKLTMQLPEDVLTQKRDAEQLWQQYMAERRNVEEYYKWPGSSTGSAESASVYDHTVVELAPGVYSGHRGTSAIESNCVDDSNDGAHGVVQAARLPVPPPKTRPPPPRNPLEHIKYQQRSVLSKAVIQLGYFPNITTTAPRFTKADDVPRPVHPDEIEGPWEVRVTYDAKDGLAYVQSLSLTSIDGAAVLSVEEEFPAAAQPYAAVDPVYQEAVRREMAQEETLMKWPNVPKWKYQYDLYTKKHLAQVVQYNYSNVVDYVDREVLLTGRSVWESPIDIDPTCGGMKSVPAHAKKPKRYMTHGLAEVGVTDI;> MRRCVMAKGEDPAHVAGWDDRQDAVEWWWTEANDSRGRQRLEAAAAVAAAAASSTVGLPLFPRFSPGRRRRRRPPAPPPPPPPLFLSRHLHSMPWLWCTCVKMQMYYTPTALTCPLSNSLAAHVGHIIVGVAALLPYSMLLFLTVMCNPRKHEPVLRAQRIRWLTFHSLMFRLLRCITASPAVAASVAVAAAQTPTSLRPAAVCRRGVHLAPSVLAASAPPPPPQQQQQPTSAAVPASTATSTTTIAAGPYRRVGNVFIVTCIDHPFKFSWEVNRMLRELRLEFMGQTTVVPDIPPVRKRIWRVRHVVRVDQLDLDEAKALIGIPEHISFRDLAGQIPPTFGRGGSVANPHMRSKMNFMRLRRMRLRDVMHRDQLEKRLLEERHHALQQQQQQQQGGGEAAAAAAATTA;> MLQRTTLRCYSALVGQATPVLLGSKGGTPKRKKNPMQLRRKTYGLHFKERYLKLEEWYFCPLCAEPKKQGEWCRREDCRQIKP;> AAAAAAAAAAAAAAAAAAAAAAAAAAAAAAAAAAAAAAAAAAAAAA;> AAAAAAAAAAAAAAAAAAAAAAAAAAAAAAAAAAAAA;> AAAAAAAAAAAAAAAAAAAAAAAAAAAAAAAAAAAAAAAAAAAAAAAAAAAAAAAAAAAAAAAAAAAAAAAAAAA;> AAAAAAAAAAAAAAAAAAAAAAAAAAAAAAAAAAAAAAAAAAAAAAAAAAAAAAAAAAAAAAAAAAAAAAAAAAAAAAAAAAAAAAAAAAAAAAAAAAAAAAAAAAAAAAAAAAAAAAAAAAAAAAAAAAAAAAAA;> AAAAAAAAAAAAAAAAAAAAAAAAAAAAAAAAAAAAAAAAAAAAAAAAAAAAAAAAAAAAAAAAAAAAAAAAAAAAAAAAAAAAAAAAAAAAAA;> AAAAAAAAAAAAAAAAAAAAAAAAAAAAAAAAAAAAAAAAAAAAAAAAAAAAAAAAAAAAAAAAAAAAAAAAAAAAAAAAAAAAAAAAAAAAAAAAAAAAAAAAAAAAAAAAAAAAAAAAAAAAAAAAAAAAAAAAAAAAAAAAAAAAAAAAAAAAAAAAAAAAAAAAAAAAAAAAAAAAAAAAAAA;> AAAAAAAAAAAAAAAAAAAAAAAAAAAAAAAAAAAAAAAAAAAAAAAAAAAAAAAAAAA;> AAAAAAAAAAAAAAAAAAAAAAAAAAAAAAAAAAAAAAAAAAAAAAAAAAAAAAAAAAAAAAAAAAAAAAAAAAAAAAAAAAAAAAAAAAAAAAAAAAAAAAAAAAAAAAAAAAAAAAAAAAAAAAAAAAAAAAAAAAAAAAAAAAAAAAAAAAAAAAAAAAAAAAAAAAAAAAAAAAAAAAAAAAAAAAAAAAAAAAAAAAA;> MFRISLICFPKAGCEEITRQGRRVVLKPQEYFAQHRMQVWQMRFKEMGPPFSRVWVALGGKMRRRRIGRQIDVKDMRYYWRPIEPQYQRLYMSRLRIKDHSNKRVQPMRLRATNNDIGQASSLKEWERSSDRKYGAALAPPKKRDFEFRVF;> MLWCTGPRRIVFHNAPSVYPFTKPFHDTPYDQDRGRFDKTKNILRENKWPAWMDHGADGTGFGIGLNRTHPLSKLRGNLRRNPSEIPRVLNMMIQGVWHKSGNKLYFRGGKPPNPSTHPYLTGEPCPVYGWKVTDPGVIREFNLPQPEDKTRYKPYVALQERKIMGMQAPTKEHSAASTSAASTDSKPLMKRLFFWK[[N'-(2,5-DIAMINO-6-HYDROXY-PYRIMIDIN-4-YL)-UREAYL]-PHEN-4-YL]-CARBONYL-GLUTAMIC ACID | C17 H19 N7 O7 | 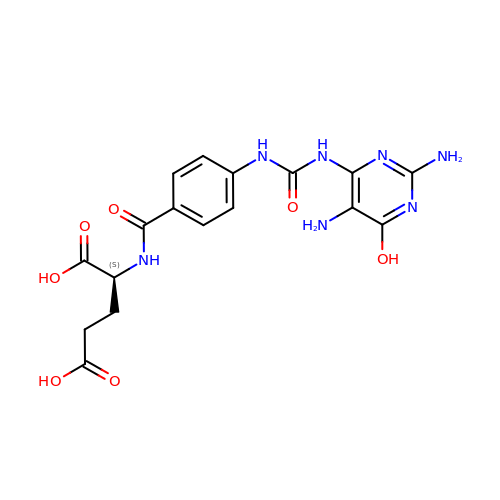SZHRIPFGZWWRKW-VIFPVBQESA-N>VSTQNEPHRFPPDFQWGVATSSYQIEGAVEADGRSPSIWDTFCARPGAIADGSTGAIANDHYHRYREDIAIMKQLGVNAYRFSIAWPRILPDGRGRVNQAGVDFYERLVDSLLEQGIEPYATLYHWDMPQVQHDRTPWYDRGVVDAFVEYTDVITRRLSDRVKYWMTLNEPWVISFLGYGAGEHAPGLRDKELYLRAAHHVLLAHGKAMPVIRANGNAQTKAGIVLNLNWVNAASDSPEDQAAARRYDQFFNRWFAEPLYNGRYPEELLEWYGRDLVPVQPGDFDIITTPTDFLAVNYYARTTVKAGSTDPMLQVDFVRPPGEYTAMDWEVYPQGLYNILNWLHTDYAPPALYVTENGAAYDDQVSAAGEVDDPQRLAYLEGHFEAAYRAIQAGIPLKGYFVWSLMDNFEWGRGFEKRFGIVFVDYATQQRIIKRSGKWFSQVTRAN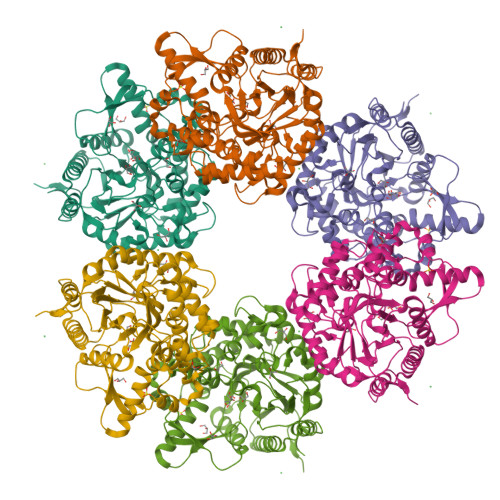GLPAPQTTLE[2x]> MELKNSISDYTEAEFVQLLKEIEKENVAATDDVLDVLLEHFVKITEHPDGTDLIYYPSDNRDDSPEGIVKEIKE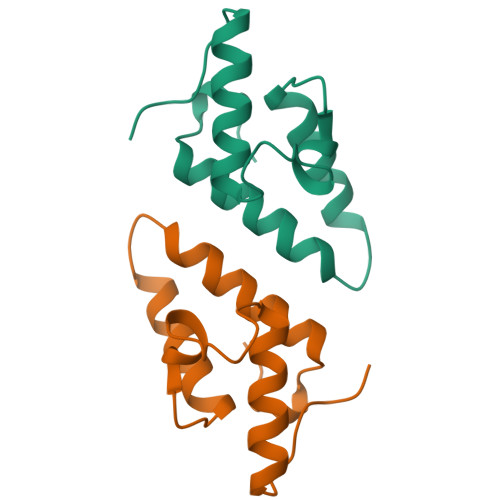WRAANGKPGFKQGKPGFKQG> CPPRHFKVGTMSSCSPWLKCPEIRSGVRRVKLIGQGAVKKVYLSEWQGQKVALSVLSSDQYADDFLHGLSMLRALQSSHVVTLVGVCEEDAVFVTEYHPLGSVLTLDTTLAQERYRWRNSWHTRLQLAIDYVAFLAYLHSSPAGIRVMCDSNDLHKTLSQFLLASDMRLLANDLDALPEVEKGGLGVKCGHHELTGDFVAPEQLWPYGEDFSFSDEAMPGYDEKTDIWKIPDVTRFLLGDVLGGDVIHFHLFQIYSECKRKEAHMRPTAREVLSVYRSVYDSMMESQSQR

On the other hand, protein O-mannose kinase (POMK, previously referred to as SgK196) is a carbohydrate kinase like Fam20B, and plays a critical role for the biosynthesis of functional α-dystroglycan (α-DG). The mannose is then phosphorylated by POMK at the C6 hydroxyl position, to allow further glycan elongation by enzymes including Fukutin, FKRP, TMEM5, B4GAT1, and LARGE. POMK mutations cause a spectrum of congenital and limb-girdle muscular dystrophies, including the most severe presentation known as the Walker-Warburg syndrome, which is associated with brain and eye abnormalities and death in early childhood. Despite compelling biochemical evidence in support of the kinase activity of POMK, its catalytic mechanism was puzzling, since it was long considered a pseudokinase.

We crystallized DrPOMK kinase domain and determined its structure in complex with Mg/ADP, aluminum fluoride, and GalNAc-β3-GlcNAc-β4-Man at 2.0 Å resolution. DrPOMK kinase has a bilobal architecture characteristic of EPKs, and can be superimposed onto PKA with a rmsd (root-mean-square difference) of 3.1 Å over 222 aligned Cα atoms. The critical role of this Lys in DrPOMK is instead served by Lys91DrPOMK located at the beginning of strand β2 that reaches into the active site and interacts with the phosphate groups of ADP. Compared to PKA, the linkers between helices αE and αF are much longer in POMK, and the catalytic Asp (Asp202DrPOMK) is located in a MCD motif in POMK. In POMK, the MCD Cys (Cys201DrPOMK) forms a disulfide bridge with the Cys in the activation segment (Cys241DrPOMK). A DLD motif is present in POMKs, and the first Asp (Asp225DrPOMK) adopts a similar position as Asp184PKA. Gln212DrPOMK at the C-terminal end of αCL occupies the position of Asn171PKA, and functions as the second metal-binding residue. The trisaccharide is nestled in a groove next to the nucleotide-binding pocket. The most prominent interaction between the mannose residue and DrPOMK is seen between the Man-O6 hydroxyl group (the phosphoacceptor) and a carboxylate oxygen of Asp202DrPOMK, the catalytic Asp. The planar AlF3 group is sandwiched between the β-phosphate of ADP and the Man, and is 1.9 Å from both the ADP donor oxygen and Man-O6, mimicking the catalytic transition state.Cytidine triphosphate synthase (CTPS) catalyzes the final and rate-limiting step of de novo CTP biosynthesis, in which a UTP is converted into CTP with the consumption of an ATP and a glutamine. A CTPS protein comprises two domains, the N-terminal ammonia ligase (AL) domain and the C-terminal glutamine amidotransferase (GAT) domain. While the active site at the AL domain activates UTP by phosphorylation using ATP to generate an iminophosphate intermediate that can react with ammonia to yield CTP, the GAT domain mediates the hydrolysis of glutamine to yield NH3 with GTP as allosteric activator. The nascent ammonia is delivered through an “ammonia tunnel,” which connects the active sites at both domains, to complete the reaction.

To reveal the structure of dmCTPS bound by all ligands without completing the reaction (dmCTPS+Sub), we used DON as a glutamine substitute for cryo-EM. We selected 424,195 particles of full-length dmCTPS in the mixture of 10 mM Mg2+, 2 mM ATP, 2 mM UTP, 2 mM GTP, and 6 μM DON. In our dmCTPS+Sub model, the binding mode of DON shows high consistency with glutamine binding in prokaryotic CTPS models, and the covalent bond between Cys399 and DON is observed, indicating that the glutamine binding site is active for the reaction of the thiol nucleophile. The GTP binding site is located at a cleft between the GAT and AL domain, which is similar to the predicted GTP binding position in ecCTPS. At the GTP binding site, the guanine base of GTP interacts with Leu444 of the binding monomer and Leu107 of another monomer through dispersion interactions and forms three hydrogen bonds with the side chain of Arg481. Yet, stabilized by the interaction between Leu444 and GTP, the wing is rather rigid in our dmCTPS+Sub map. However, when GTP is positioned at the binding site, the cleft between the glutaminase active site and the ammonia tunnel is fully covered by GTP, suggesting that GTP serves as a block to prevent molecules shuttling between the interior and exterior spaces of the protein. In our dmCTPS+Sub map, we observe additional electron density merging with the uracil base in the direction of the 4-oxygen atom, which would be phosphorylated in the reaction. Meanwhile, the signal of the γ-phosphate of ATP is missing, suggesting that the reaction of UTP phosphorylation is taking place in our imaging condition. We further focused on residues participating in this transformation and identified Lys16 and Lys38 directly interact with transferred phosphate and Asp70 and Glu145 also interact through a water molecule, supporting previous predictions about their function of stabilizing the anionic transition state during the reaction.

>[4x]MKYILVTGGVISGVGKGVIASSFGTLLKSCGLDVTSIKIDPYINIDAGTFSPYEHGEVYVLDDGAEVDLDLGNYERFLDVTLHRDNNITTGKIYKLVIEKERTGEYLGKTVQVVPHITDAIQEWVERVAQTPVQGSSKPQVCIVELGGTIGDIEGMPFVEAFRQFQFRVKRENFCLAHVSLVPLPKATGEPKTKPTQSSVRELRGCGLSPDLIVCRSEKPIGLEVKEKISNFCHVGPDQVICIHDLNSIYHVPLLMEQNGVIEYLNERLQLNIDMSKRTKCLQQWRDLARRTETVRREVCIAVVGKYTKFTDSYASVVKALQHAALAVNRKLELVFIESCLLEEETLHSEPSKYHKEWQKLCDSHGILVPGGFGSRGMEGKIRACQWARENQKPLLGICLGLQAAVIEFARNKLGLKDANTTEIDPNTANALVIDMPEHHTGQLGGTMRLGKRITVFSDGPSVIRQLYGNPKSVQERHRHRYEVNPKYVHLLEEQGMRFVGTDVDKTRMEIIELSGHPYFVATQYHPEYLSRPLKPSPPFLGLILASVDRLNQYIQRGCRLSPRQLSDASSDEEDSVVGLAGATKSLSSLKIPITPTNGISKSCNGSISTSDSEGACGGVDPTNGHK> GPLGSPEFPGRLAAGVDCGDGVGARQHVFLVSEYLKDASKKMKNGLMFVKLVNPCSGEGAIYLFNMCLQQLFEVKVFKEKHHSWFINQSVQSGGLLHFATPVDPLFLLLHYLIKADKEGKFQPLDQVVVDNVFPNCILLLKLPGLEKLLHHVTEEKGNPEIDNKKYYKYSKEKTLKWLEKKVNQTVAALKTNNVNVSSRVQSTAFFSGDQASTD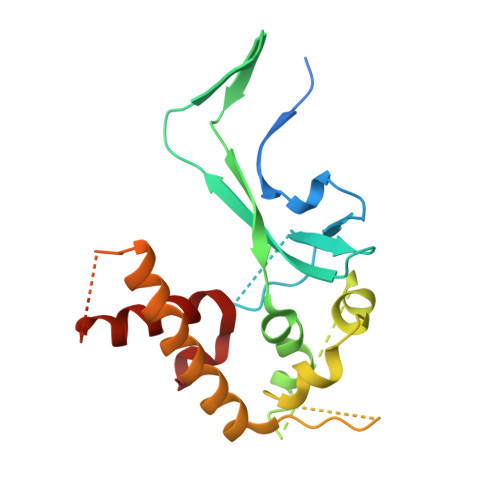KEEDYIRYAHGLISDYIPKELSD>[2x]MPFVKGFEPISLRDTNLFEPIKIGNTQLAHRAVMPPLTRMRATHPGNIPNKEWAAVYYGQRAQRPG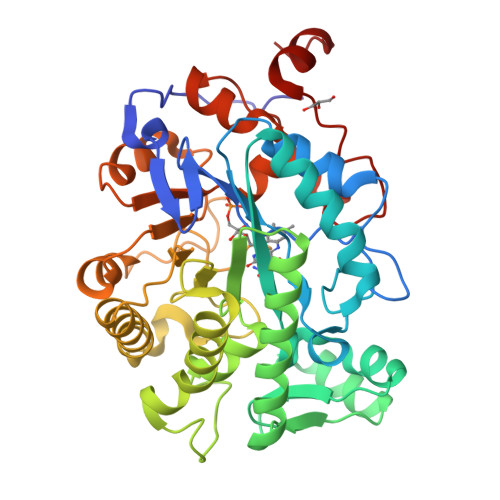TMIITEGTFISPQAGGYDNAPGIWSDEQVAEWKNIFLAIHDCQSFAWVQLWSLGWASFPDVLARDGLRYDCASDRVYMNATLQEKAKDANNLEHSLTKDDIKQYIKDYIHAAKNSIAAGADGVEIHSANGYLLNQFLDPHSNKRTDEYGGTIENRARFTLEVVDALIETIGPERVGLRLSPYGTFNSMSGGAEPGIIAQYSYVLGELEKRAKAGKRLAFVHLVEPRVTDPSLVEGEGEYSEGTNDFAYSIWKGPIIRAGNYALHPEVVREQVKDPRTLIGYGRFFISNPDLVYRLEEGLPLNKYDRSTFYTMSAEGYTDYPTYEEAVDLGWNKN>[6x]GGGGUTTGGG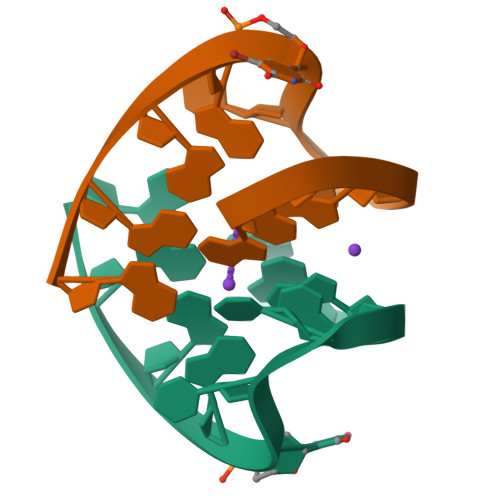G> MAGGIGNKGDYIITYRGDTRSFTEIFDKGFETLGPSKDLYKHALDNRAPPSDFVSTTIDPTKTISFATKYGQKSGYMYTMKTNHGIDVNKALGARSPFAAEAEIAMPGGVR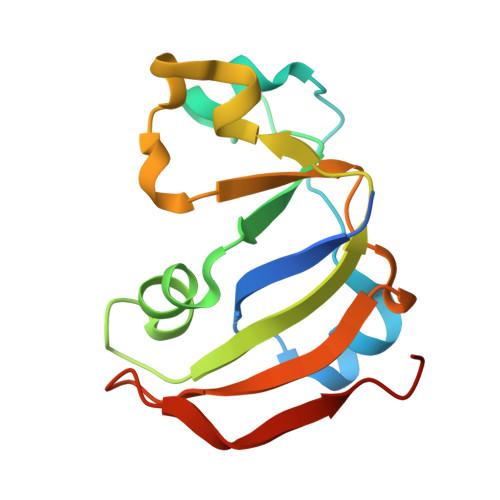AEDILGARAVNADGEMWDYTILNPKRYGK> GPLGSHMSVYPKALRDEYIMSKTLGSGACGEVKLAFERKTCKKVAIKIISKRKFAIGSAREADPALNVETEIEILKKLNHPCIIKIKNFFDAEDYYIVLELMEGGELFDKVVGNKRLKEATCKLYFYQMLLAVQYLHENGIIHRDLKPENVLLSSQEEDCLIKITDFGHSKILGETSLMRTLCGTPTYLAPEVLVSVGTAGYNRAVDCWSLGVILFICLSGYPPFSEHRTQVSLKDQITSGKYNFIPEVWAEVSEKALDLV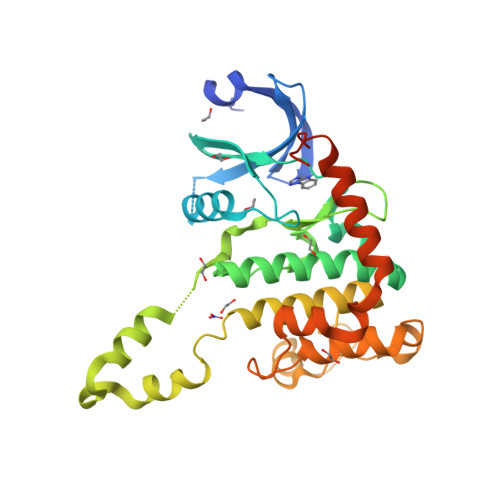KKLLVVDPKARFTTEEALRHPWLQDEDMKRKFQDLLSEENESTALPQVLAQPSTSRKRPREGEAEGAE>SQNRVPSSRTVSYFVAKPSSSEMEKLQLGPEDSILRMERIRFADDIPICFEVASIPYSLVSQYGKSEITNSFYKTLEAKSGHKIGHSNQTISAVQASEQIAEYLEIKRGDAILRVRQVSYFENGLPF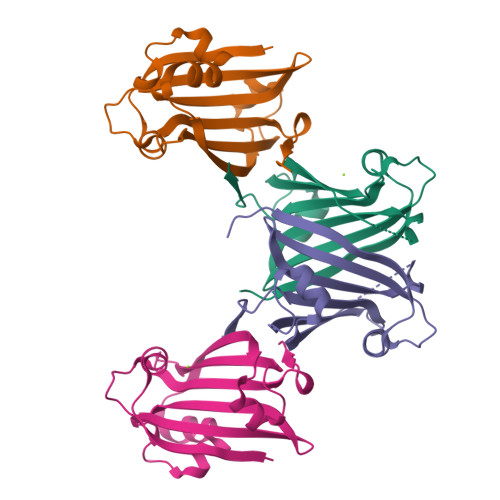EYVRTQYAGSRFEFYLEK[4x]> MQKHWWHKATVYQIYPKSFMDTNGDGIGDLKGITSKLDYLQKLGVMAIWLSPVYDSPMDDNGYDIANYEAIADIFGNMADMDNLLTQAKMRGIKIIMDLVVNHTSDEHAWFIEAREHPDSSERDYYIWCDQPNDLESIFGGSAWQYDDKSDQYYLHFFSKKQPDLNWENAN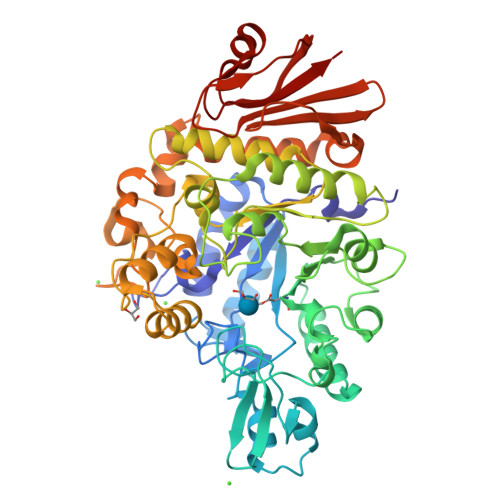LRQKIYDMMNFWIDKGIGGFRMDVIDMIGKIPAQHIVSNGPKLHAYLKEMNAASFGQHDLLTVGQTWGATPEIAKQYSNPVNHELSMVFQFEHIGLQHKPEAPKWDYVKELNVPALKTIFNKWQTELELGQGWNSLFWNNHDLPRVLSIWGNTGKYREKSAKALAILLHLMRGTPYIYQGEEIGMTNYPFKDLNELDDIESLNYAKEAFTNGKSMETIMDSIRMIGRDNARTPMQWDASQNAGFSTADKTWLPVNPNYKDINVQAALKNSNSIFYTYQQLIQLRKENDWLVDADFELLPTADKVFAYLRKVREERYLIVVNVSDQEEVLEIDVDKQETLISNTNESAALANHKLQPWDAFCIKIL> KA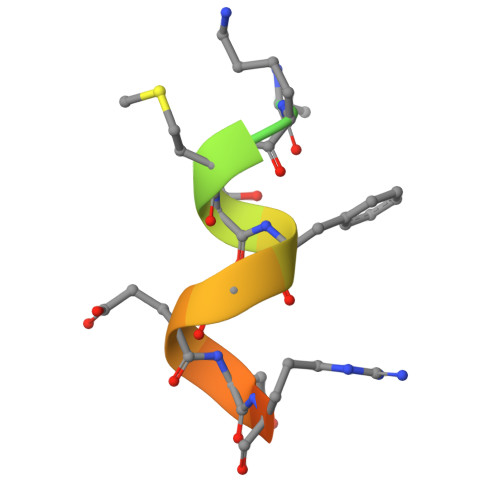HTSVKKMTFGENRDLER7-cyclopentyl-N,N-dimethyl-2-{[5-(methylcarbamoyl)pyridin-2-yl]amino}-7H-pyrrolo[2,3-d]pyrimidine-6-carboxamide | C21 H25 N7 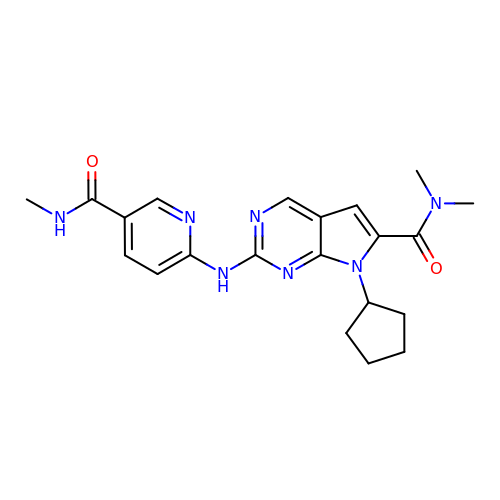O2 | ZWAGHYMVHPAUMT-UHFFFAOYSA-N>SNAMTLVYQSTRDANNTVTASQAILQGLATDGGLFTPDTYPKVDLNFDKLKDASYQEVAKLVLSAFLDDFTVEELDYCINNAYDSKFDTPAIAPLVKLDGQYNLELFHGSTIAFKDMALSILPYFMTTAAKKHGLENKIVILTATSGDTGKAAMAGFANVPGTEIIVFYPKDGVSKIQELQMTTQTGDNTHVIAIDGNFDDAQTNVKHMFNDVALREKLTTNKLQFSSANSMNIGRLVPQIVYYVYAYAQLVKTGEIVAGEKVNFTVPTGNFGNILAAFYAKQIGLPVGKLICASNDNNVLTDFFKTRVYDKKREFKVTTSPSMDILVSSNLERLIFHLLGNNAEKTTELMNALNTQGQYKLTDFDAEILDLFAAEYATEEETAAEIKRVCELDSYIED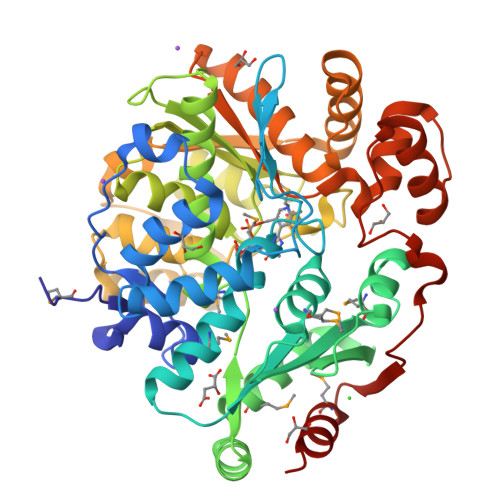PHTAVASAVYKKYQSATGDVTKTVIASTASPYKFPVVAVEAVTGKAGLTDFEALAQLHEISGVAVPPAVDGLEIAPIRHKTTVAAADMQAAVEAYLGL[2x]Cell-surface expressed contactin 1 and neurofascin 155 control wiring of the nervous system and interact across cells to form and maintain paranodal myelin-axon junctions. Defining subfamily features are extracellular six N-terminal immunoglobulin-like domains (Ig), four fibronectin type III domains (FnIII) and posttranslational modifications, i.e., N-glycosylation at multiple sites and a C-terminal glycophosphatidylinositol (GPI)-membrane anchor. All four members are type I transmembrane proteins with six extracellular N-terminal Ig like domains, three to five FnIII domains, various predicted N-glycosylation sites, a single transmembrane spanning helix, and a ∼120 cytoplasmic region with a highly conserved ankyrin binding sequence. To address these questions, we structurally characterized the contactin 1 and neurofascin 155 interacting regions, i.e., Ig1–Ig6, individually and in complex.

The Ig5–Ig6 combination orients away but nearly in plane with the Ig1–Ig4 horseshoe in a curved architecture giving the molecule a sickle-like shape, with Ig1–Ig4 forming the “handle” and Ig5–Ig6 the curved “blade”. Contactin 1 Ig1–Ig4 horseshoe segment resembles previously reported contactin 1, 2, 4 and 5 segments. Contactin 1 forms a larger-order zipper in the crystal that is also formed in solution and the neurofascin 155 binding site is exposed in this oligomer. The zipper arrangement emerges from four interfaces, denoted α to δ, that capture four separate dimeric arrangements of constituting chains. The dimer burying most surface area buries 2980 Å2 and does so using twice the interface α where Ig3–Ig4 on one molecule contact Ig6 of the other molecule. The second dimeric arrangement involves interface β burying 1190 Å2 through Ig3–Ig3 interactions between chain A and a symmetry related chain B. In interface γ, Ig3 of chain A contacts Ig5–Ig6 of a symmetry related equivalent molecule, whereas interface δ forms by Ig6–Ig6 interactions between chain B and a symmetry related chain A. Addition of a contactin 1 molecule to a dimer formed through interface α to form a trimer, contributes two additional interaction interfaces, e.g., β and γ. In particular the glycans on Asn258 of Ig3 and Asn521 of Ig6 are located close to intermolecular interaction sites and may influence interactions depending on their composition. Contactin 1 may however form cis interactions, and the zipper is compatible with cis-interactions as the c-termini, that connect to the cell surface, are all on the same side. While contactin 1 and neurofascin 155 interact in a mode similar as to neurofascin30 and contactin 222 homodimerization, in the structure we report contactin 1 does not form homodimers via the Ig1–Ig2 interface.

>GSDFTWHRRYGHGVSEEDKGFGPIFEEQPINTIYPEESLEGKVSLNCRARASPFPVYKWRMNNGDVDLTNDRYSMVGGNLVINNPDKQKDAGVYYCLASNNYGMVRSTEATLSFGYLDPFPPEERPEVKVKEGKGMVLLCDPPYHFPDDLSYRWLLNEFPVFITMDKRRFVSQTNGNLYIANVESSDRGNYSCFVSSPSITKSVFSKFIPLIPIPERTTKPYPADIVVQFKDIYTMMGQNVTLECFALGNPVPDIRWRKVLEPMPSTAEISTSGAVLKIFNIQLEDEGLYECEAENIRGKDKHQARIYVQAFPEWVEHINDTEVDIGSDLYWPCIATGKPIPTIRWLKNGYSYHKGELRLYDVTFENAGMYQCIAENAYGSIYANAELKILALAPTFEMNPMKKKILAAKGGRVVIECKPKAAPKPKFSWSKGTEWLVNSSRILIWEDGSLEINNITRNDGGIYTCFAENNRGKANSTGTLVITNPTRIILAPINADITVGENATMQCAASFDPALDLTFVWSFNGYVIDFNKEITHIHYQRNFMLDANGELLIRNAQLKHAGRYTCTAQTIVDNSSASADLVVRGHHHHHH[2x]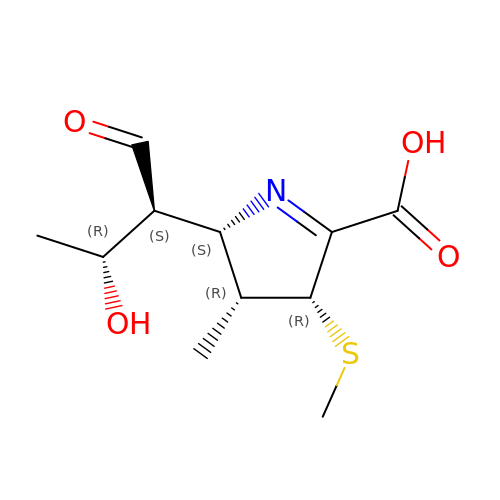(2S,3R,4R)-2-[(2S,3R)-3-hydroxy-1-oxobutan-2-yl]-3-methyl-4-(methylsulfanyl)-3,4-dihydro-2H-pyrrole-5-carboxylic acid | C11 H17 N O4 S | ASUOZXIKIDLJND-VRRGKTLJSA-N>[2x]MSQEVIRGIALPPAAQPGDPLARVDTPSLVLDLPAFEANLRAMQAWADRHEVALRPHAKAHKCPEIALRQLALGARGICCQKVSEALPFVAAGIRDIHISNEVVGPAKLALLGQLARAAKISVCVDNAENLAQLSAAMTRAGAEIDVLVEVDVGQGRCGVSDDATVLALAQQARALPGLNFAGLQAYHGSVQHYRTREERAAVCRQAARIAASYAQLLRESGIACDTITGGGTGSVEFDAASGVY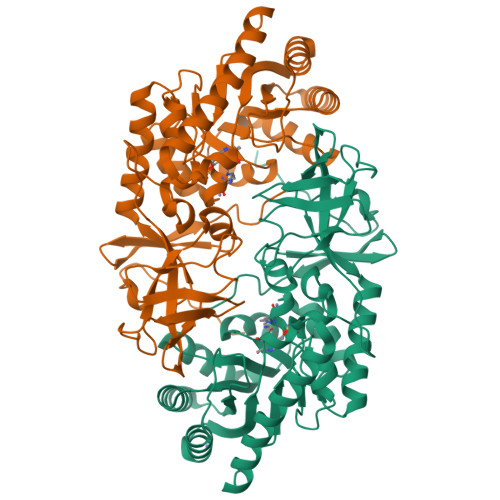TELQAGSYAFMDSDYGANEWNGPLKFQNSLFVLSTVMSTPAPGRVILDAGLKSTTAECGPPAVYGEPGLTYAAINDEHGVVRVEPGAQAPALGAVLRLVPSHVDPTFNLHDGLVVVKDGVVQDVWEIAARGFSR>[4x]KDKKKGKKNIPMTEIQTTGTQDRAIWVKLLWKISY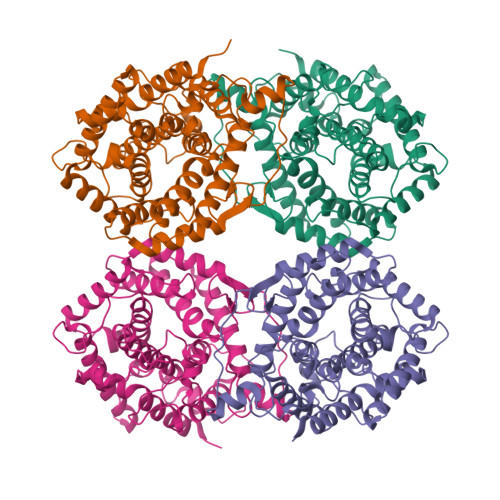PVIHNLAEGTLHQNMPIETRSGETAGYKDMTHLEAVGRTLAGVAPWLALPDDDTEEGKLRKQMREEVLKGLKNAVDPASPDLLNFTKHAQPIVDAAYLVHAFLRAPKALWEPLDEVTKERYIKSFQSLRDRTGAYNNWLLFTGLTESFLLGKGVQYDQFRIRVSKNKVKEWYVGDGWYSDGPSFSMDNYNAYVMHSMMVAMLENLLPKRWASQKELDEAMNRMIRHSEFCERMIAPDGTYPAFGRSVTYRTAAFQSLADVALRKKLPSHVSPAQVRCALTAVHRNMYEGNQNFDKDGWLVLGFNGHQPECADGYTSTGSLYMATLSFLPLGLPADDPFWTDAYADWTSKKAWKGGHLHKDYKVEY>[2x]GPHMLEREKIYQWINELSSPETRENALLELSKKRESVPDLAPML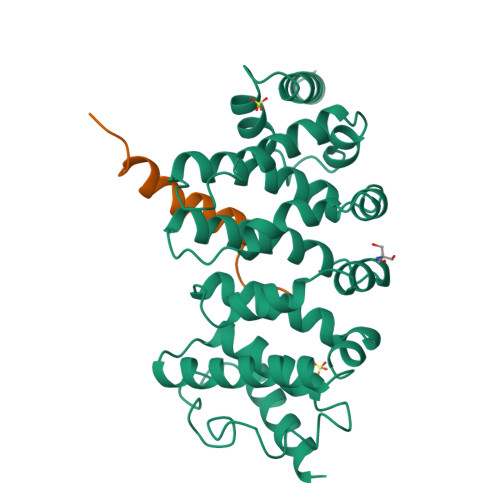WHSFGTIAALLQEIVNIYPSINPPTLTAHQSNRVCNALALLQCVASHPETRSAFLAAHIPLFLYPFLHTVSKTRPFEYLRLTSLGVIGALVKTDEQEVINFLLTTEIIPLCLRIMESGSELSKTVATFILQKILLDDTGLAYICQTYERFSHVAMILGKMVLQLSKEPSARLLKHVVRCYLRLSDNPRAREALRQCLPDQLKDTTFAQVLKDDTTTKRWLAQLVKNLQE;>DDDLGFDPFVETQKGLAELMENEVVQ[2x]>[2x]MGHHHHHHGGHMSLLTFVGLGLWDVKDISVKGLEAVREADEVYVEYYTSKLLSSIEEMEEFFGKRVVELERSDLEENSFRLIE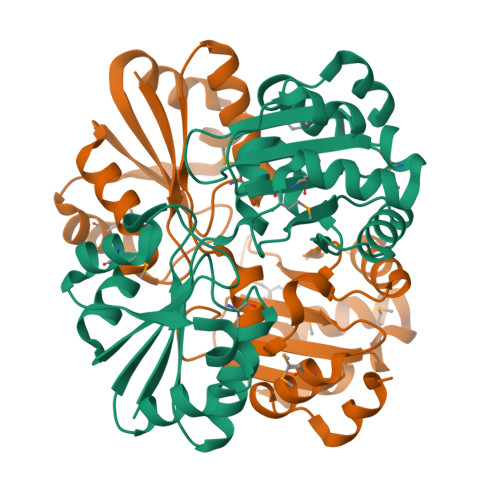RAKSKSVVLLVPGDPMVATTHSAIKLEAERKGVKTRIIHGASISTAVCGLTGLHNYRFGKSATVSWHRSQTPVNVIKANRSIDAHTLLFLDLHPEPMTIGHAVENLIAEDAQMKDLYAVGIARAGSGEEVVKCDRLENLKKIDFGKPLHVMVVLAKTLHFMEFECLREFADAPAELERLVAEGGS>[2x]XAAALAAALA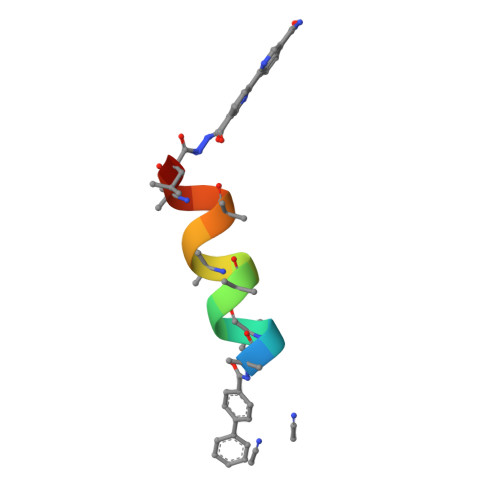QALX>[2x]MAHHHHHHMLHNTFFICETNQIMNEIEKAKGIILNRNMNDIWSALLIEVKKSNLIIKSTDRNIFFESTISIVSETDFKVLINASNFYDAVKAFNFYKKIKIVFNENNSKLEIMGELNDEKEEYEDHLKEPTFSYEEIENYNYDMVNEDYTFGIEIKQKSFKKVINRIAFSAHLDESKNVLNGVYFSKDEDSKLLLVSTN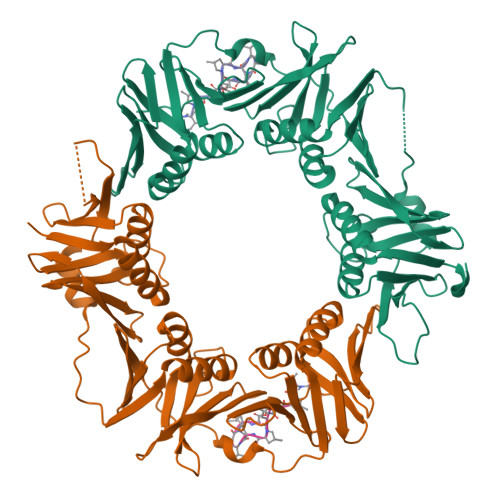GHRMSICKTEVIVEEDVNFIVPVKIFNFLKHLMSGEGMVKIKFSDKKFYVEFDNYKIACSLINGNYPDYKSIIPKEQKNKSLVSLGILKDRLARVNLYVDKSRKLVLTFSELQLKLLGEDLITGRKGEFFIKDPNYLYDGADEVMAINISYFVEAISVFETSKIEIQFNSGNVLKLSEPENFNFTHLIMPMSLG;>[2x]XVPTLPLVPXG> MCWAAAIPIAISGAQAISGQNAQAKMIAAQTAAGRRQA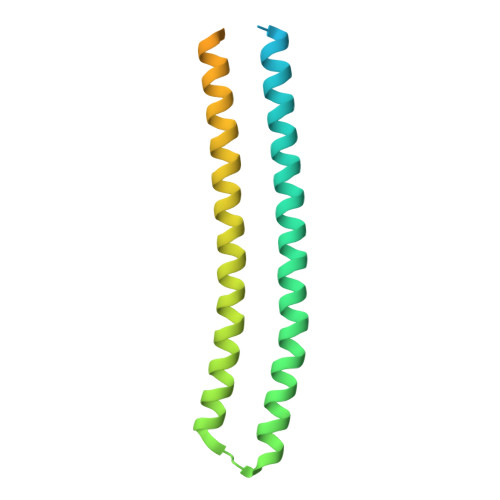MEIMRQTNIQNADLSLQARSKLEEASAELTSQNMQKVQAIGSIRAAIGESMLEGSSMDRIKRVTEGQFIREANMVTENYRRDYQAIFAQQLGGTQSAASQIDEIYKSEQKQKSKLQMVLDPLAIMGSSAASAYASGAFDSKSTTKAPIVAAKGTKTGR>[2x]GHMNQYIYPEIQRSQIFYCNHMGREPGVFKSSFFNYSEIKKGFQFKVIQEKLQGRQFINSDKIKPDHPQTIIKKTLLKEYQSKNFSCQEERDLFLEFTEKIVQNFHNINFNYLLKKFCKLPENYQSLKSQVKQIVQSENKANQQSCENLFNSLYDTEISYK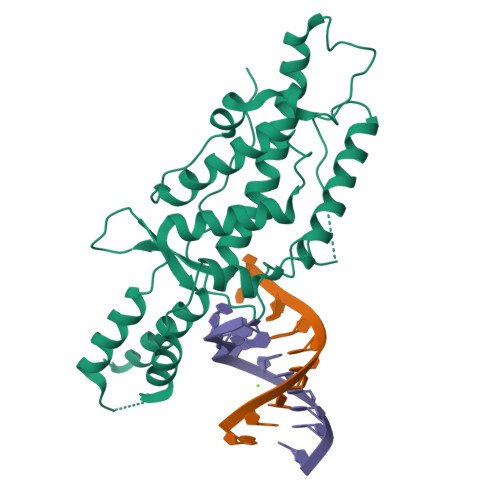QITNFLRQIIQNCVPNQLLGKKNFKVFLEKLYEFVQMKRFENQKVLDYICFMDVFDVEWFVDLKNQKFTQKRKYISDKRKILGDLIVFIINKIVIPVLRYNFYITEKHKEGSQIFYYRKPIWKLVSKLTIVKLEEENLEKVE>GSHMAPLKDVYKNDFLIGNAISAEDLEGTRLELLKMHHDVVTAGNAMKPDALQPTKGNFTFTAADAMIDKVLAEGMKMHGHVLVWHQQSPAWLNTKKDDNNNTVPLGRDEALDNLRTHIQTVMKHFGNKVISWDVVNEAMNDNPSNPADYKASLRQTPWYQAIGSDYVEQAFLAAREVLDENPSWNIKLYYNDYNEDNQNKATAIYNMVKDINDRYAAAHNGKLLIDGVGMQGHYNINTNPDNVKLS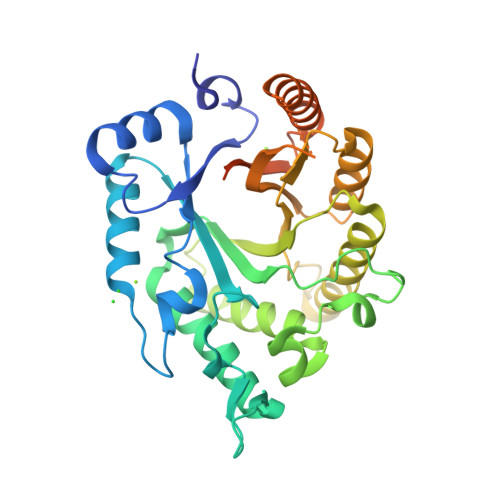LEKFISLGVEVSVSELDVTAGNNYTLPENLAVGQAYLYAQLFKLYKEHADHIARVTFWGMDDNTSWRAENNPLLFDKNLQAKPAYYGVIDPAEQ[2x]> LKESPSGYLRSGEGDTGCGELVWVGEPLTLRTAETITGKYGVWMRDPKPTYPYTQETTWRIDTVGTDVRQVFEYDLISQFMQGYPSKVHILPRPLESTGAVMYSGSLYFQGAESRTVIRYELNTETVKAEKEIPGAGYHGQFPYSWGGYTDIDLAVDEAGLWVIYSTDEAKGAIVLSKLNPENLELEQTWETNIRKQSVANAFIICGTLYTVSSYTSADATVNFAYDTGTGISKTLTIPFKNRYKYSSMIDYNPLEKKLFAWDNLNMVTYDIKLSKM

Inherited missense mutations in the myocilin (MYOC) gene, within its olfactomedin (OLF) domain, constitute the strongest genetic link to primary open-angle glaucoma via a toxic gain of function, and thus MYOC is an attractive precision-medicine target. Myocilin has no known function, and there is no glaucoma phenotype in Myoc knockout mice or in individuals with a homozygous N-terminal truncation mutation or hemizygous deletion of MYOC, but rare non-synonymous coding mutations lead to toxic intracellular sequestration of misfolded myocilin. However, not all mutations in MYOC cause glaucoma, and common variants are expected to be neutral polymorphisms. Among the common features associated with pathogenic myocilin misfolding, we demonstrate that a single metric, OLF thermal stability, can robustly segregate benign from early-onset disease variants.

Overall, nine variants (T256M, R296H, L303I, S313F, V329M, S331L, E352K, A427T, and V499I) were considered likely to be benign. Similarly, V329M, a substitution that occurs in the hydrophobic interior of OLF, is not sterically compatible. Previous support for the V329M variant as benign comes primarily from the observation that methionine is the corresponding residue in Danio rerio myocilin, but the mutation has also been documented among glaucoma patients, including one diagnosed with juvenile OAG. Assessment of spent media from cells expressing each of the 16 full-length myocilin variants revealed WT-like secretion for T256M, R296H, L303I, S313F, V329M, S331L, T353I, A445V, V449I and K500R. Structural integrity was further confirmed by high-resolution crystal structures, which were solved for 11 OLF variants. No gross changes from WT OLF were detected for the structures of T293K, R296H, L303I, V329M, S331L, E352K, T353I, K398R, A445V, V449I or K500R, indicating that these mutations are accommodated within the native five-bladed β-propeller fold and do not perturb the dinuclear calcium-containing site. Surprisingly, V329M does not appear to harbor any pathogenic signatures despite its location in an internal strand associated with amyloid formation and its involvement in a hydrophobic patch that is disrupted in other disease variants like W286R. In addition to the five variants that we predicted initially to be benign (T293K, T353I, K398R, A445V and K500R), our study reveals seven more (T256M, R296H, L303I, V329M, S331L, E352K and V499I) that are indistinguishable from WT OLF across multiple assays. Thus, our data indicate these should also be considered benign.>MTTGLSTAGAQDIGRSSVRPYLEECTRRFQEMFDRHVVTRPTKVELTDAELREVIDDCNAAVAPLGKTVSDERWISYVGVVLWSQSPRHIKDMEAFKAVCVLNCVTAVWDDMDPALHDFGLFLPQLRKICEKYYGPEDAEVAYEAARAFVTSDHMFRDSPIKAALCTTSPEQYFRFRVTDIGVDFWMKMSYPIYRHPEFTEHAKTS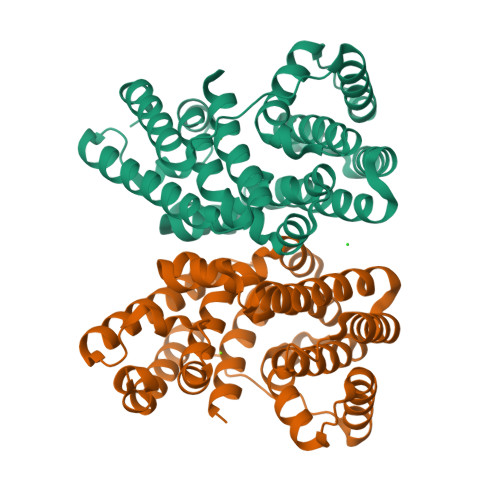LAARMTTRGLTIVNDFYSYDREVSLGQITNCFRLCDVSDETAFKEFFQARLDDMIEDIECIKAFDQLTQDVFLDLIYGNFVWTTSNKRYKTAVNDVNSRIQAAALEHHHHHH[2x]> MRGRLFTLVSCLLLSISSVDAVHAASLTEQRRLYDQAKAALAKGNSAPYMASRSALRDYPLEPYLAYDELTHRLKSASNEEVERFLTEHGDLPQIGWLKLRWLRLLADRGDWKTFVNYYDPKLNFTELDCLYGQYQLGHGQKAEGYATSERLWLVGKSQPAACDTLFGLWQGEGQLTEEKVWKRLKLAAEARNYSLASHLAQRLPTLGNQGALMVSVAQNPAQLSQTGRFSQRDHATADVVGLGLRRLARQDPEKALSLLDYYSSALPFSSDEKVAIAREIGLSLAKRFDPRALPLMTQYDPGLRDNTVTEWRTRLLLRLGRWDEAYALTRKLPQDLAATSRWRYWQARSLQLAQPNSKEPIALYQKLAGERDFYGFLAADRLSVPYKLGNRPAHIDPRVLQRVRNAASTRRAMEFFNRGEVINARREWYHAARLFDRDELIAQARLAYDMQWYFPAIRSISQAQYWDDLDIRFPMAHRATLVREAKNRGLHSSWIFAITRQESAFMSDARSGVGATGLMQLMPGTAKETSRKFGIPLASTQQLIVPDVNIRLGAAYLSQVHSQFNGNRVLASAAYNAGPGRVRQWLKDTRHLAFDVWIETIPFDETRQYVQNV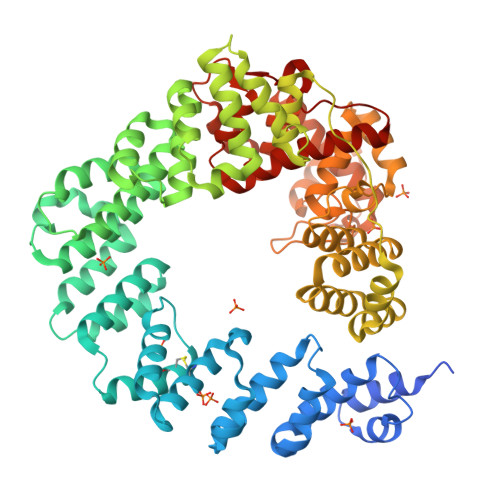LSYAVIYGQKLNAPQPIVDWHERYFDDL> MNNGEGEVMDLRDIDLNLLVVFNQLLLDRSVSTAGEKLGLTQPAVSNSLKRLRTALNDDLFLRTSKGMEPTPYALHLAEPVIYALNTLQTALTTRNSFDPFASTRTFNLAMTDIGEMYFMPPLMEALAQRAPHIQISTLRPNAGNLKEDMESGAVDLALGLLPELQTGFFQRRLFRHRYVCMFRKDHPSAKSPMSLKQFSELEHVGVVALNTGHGEVDGLLERAGIKRRMRLVVPHFIAIGPILHSTDLIATVPQRFAVRCEVPFGLTTSPHPAKLPDIAINLFWHAKYNRDPGNMWLRQLFVELFSEAHHHHHH;> MNNGEGEVMDLRDIDLNLLVVFNQLLLDRSVSTAGEKLGLTQPAVSNSLKRLRTALNDDLFLRTSKGMEPTPYALHLAEPVIYALNTLETALTTRDSFDPFASTRTFNLAMTDIGEMYFMPPLMEALAQRAPHIQISTLRPGAGNLKEDMESGAVDLALGLLPELQTGFFQRRLFRHRYVCMFRKDHPSAKSPMSLKQFSELEHVGVVALNTGHGEVDGLLER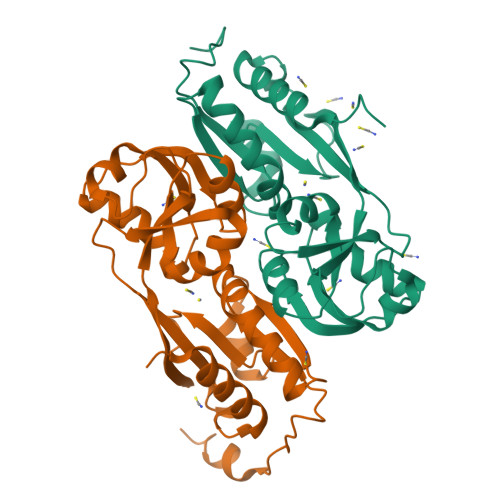AGIKRRMRLVVPHFIAIGPILHSTDLIATVPQRFAVRCEVPFGLTTSPHPAKLPDIAINLFWHAKYNRDPGNMWLRQLFVELFSEAHHHHHH>[2x]HHHHHHFNLPPGNYKKPKLLYCSNGGHFL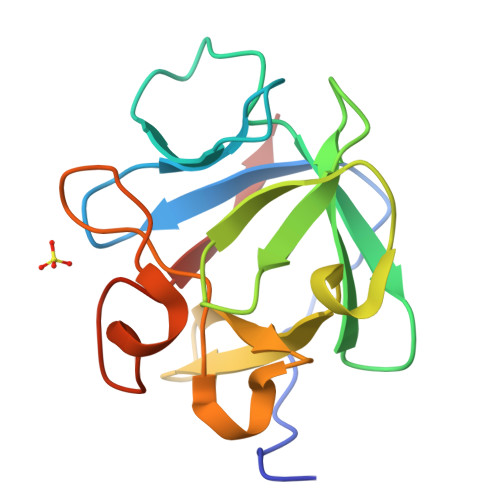RILPDGTVDGTRDRSDQHIQLQLSAESVGEVYIKSTETGQYLAMDTDGLLYGSQTPNEEVLFLERLEENHYNTYISKKHAEKNWFVGLKKNGSCKRGPRTHYGQKAILFLPLPVSSD>GSHMAKEEIIWESLSVDVGSQGNPGIVEYKGVDTKTGEVLFEREPIPIGTNNMGEFLAIVHGLRYLKERNSRKPIYSNSQTAIKWVKDKKAKSTLVRNEETALIWKLVDEAEEWLNTHTYETPILKWQTDKWGEIKADYGRK[2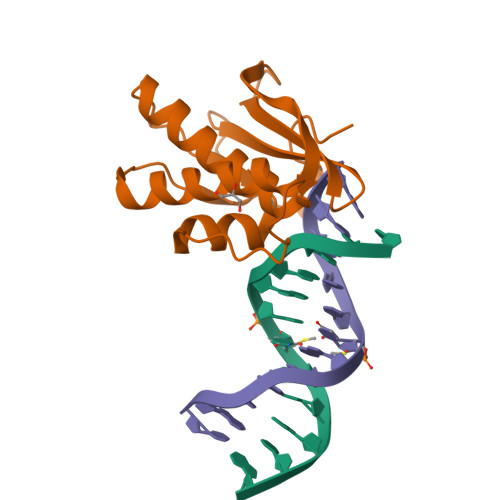x]> MSQSNRELVVDFLSYKLSQKGYSWSQFSDVEENRTEAPEETEAERETPSAINGNPSWHLADSPAVNGATGHSSSLDAREVIPMAAV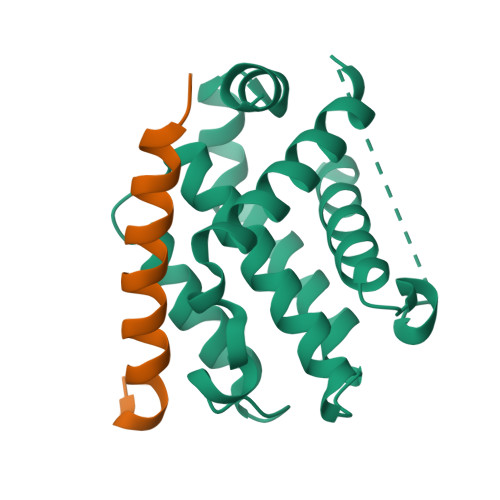KQALREAGDEFELRYRRAFSDLTSQLHITPGTAYQSFEQVVNELFRDGVNWGRIVAFFSFGGALCVESVDKEMQVLVSRIASWMATYLNDHLEPWIQENGGWDTFVDLYGNNAAAESRKGQERFN;> APPNLWAAQRYGRELRRMSDEFEGSFK>[2x]SSSHPIFHRGEFSVCDSVSVWVGDKTTATDIKGKEVMVLGEVNINNSVFKQYFFETKCRDPNPVDSGCRGIDSKHWNSYCTTTHTFVKALTMDGKQAAWRFIRIDTACVCVLSRKAVRRA;> KETCST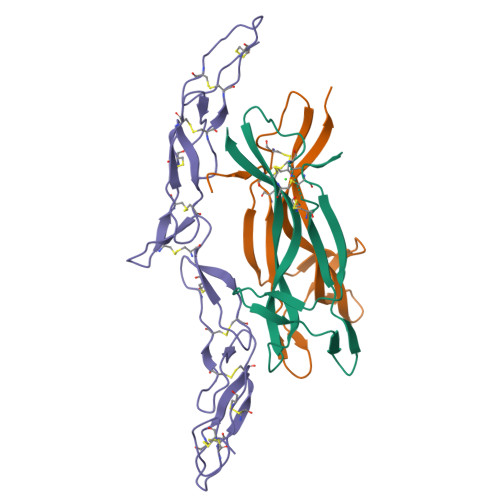GLYTHSGECCKACNLGEGVAQPCGANQTVCEPCLDNVTFSDVVSATEPCKPCTECLGLQSMSAPCVEADDAVCRCAYGYYQDEETGHCEACSVCEVGSGLVFSCQDKQNTVCEECPEGTYSDEANHVDPCLPCTVCEDTERQLRECTPWADAECE> WVQPITCQKPSLTLWLDDKMFTGLINTGADVTIIK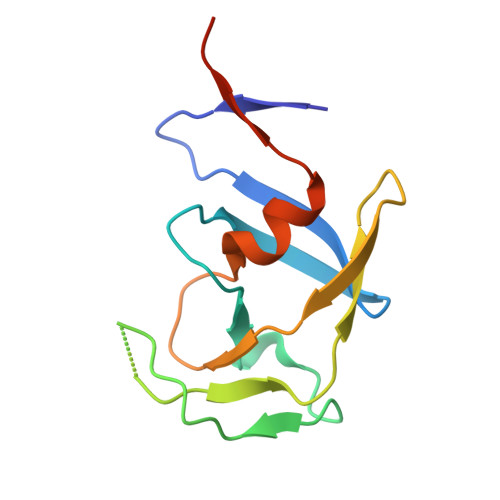LEDWPPNWPITDTLTNLRGIGQSNNPKQSSKYLTWRDKENNSGLIKPFVIPNLPVNLWGRDLLSQMKIMMCSPNDIVTA> MGSLGEEPQVAEDCMGLLQLLS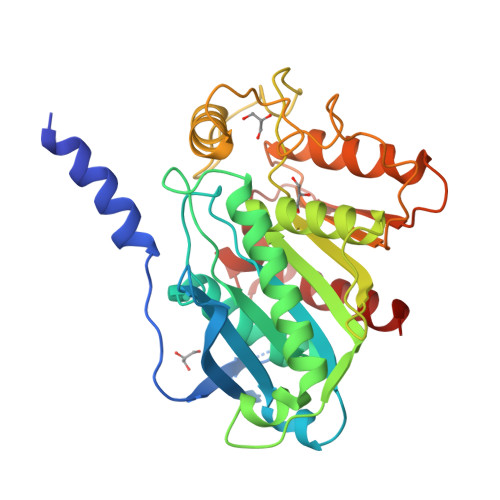NGTVLRSESIDLITQQIPFKNNQTVLFKDSIYHKPNNLHLRLYKPISASNRTALPVVVFFHGGGFCFGSRSWPHFHNFCLTLASSLNALVVSPDYRLAPEHRLPAAFEDAEAVLTWLWDQAVSDGVNHWFEDGTDVDFDRVFVVGDSSGGNIAHQLAVRFGSGSIELTPVRVRGYVLMGPFFGGEERTNSENGPSEALLSLDLLDKFWRLSLPNGATRDHHMANPFGPTSPTLESISLEPMLVIVGGSELLRDRAKEYAYKLKKMGGKRVDYIEFENKEHGFYSNYPSSEAAEQVLRIIGDFMNNLS>GMRVDSQMSNLSRREFSYLLTIKRYNDSGEGAKINRIAKDLKIAPSSVFEEVSHLEEKGLVKKKEDGVWITNNGTRSINYLIKAHRVIEILLVNIGIDKQTACEYSKQFDYLIPEEIIDKLYNYLGKPSYCPHGL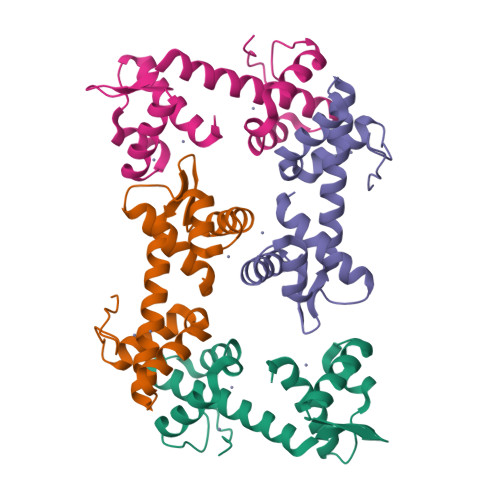EIPL[4x]> GPLGSEPRSLTA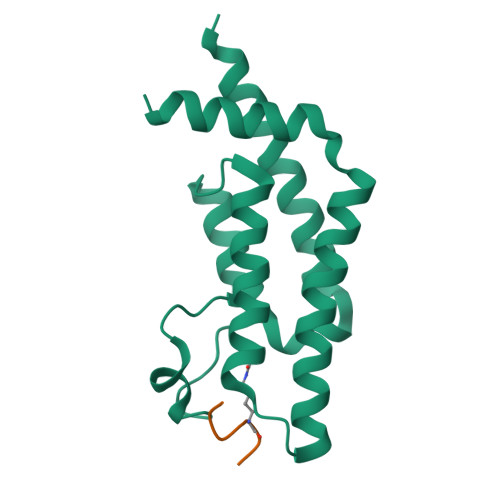EEVKRLEEQEEDTFRELRIFLRNVTHRLAIDKRFRVFTKPVDPDEVPDYVTVIKQPMDLSSVISKIDLHKYLTVKDYLRDIDLICSNALEYNPDRDPGDRLIRHRACALRDTAYAIIKEELDEDFEQLAEEIQESRKKRG;> SGRGKGGKGLGKGGA> MAHHHHHHMSLAEFALIDRIRARTLERDDILLGIGDDAALLQPRANEQLVVTADTLNSGVHFPVETRAFDIGWKTLAVNLSDLAAMGARPAWCTLALSLPEASE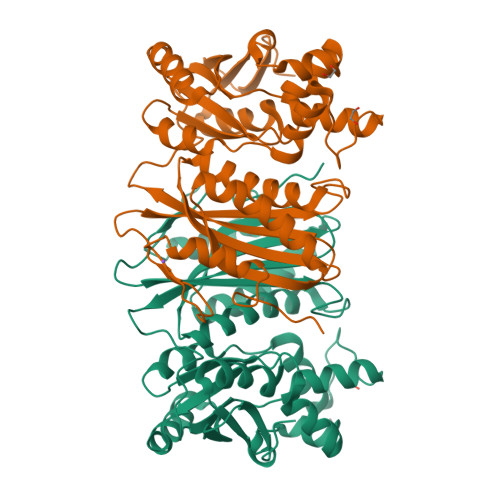DWIEAFGDGFFALADQHDIALIGGDTTRGPLSLSVTAMGQVGRGQALRRDRAQLGDDIWVSGTLGDAAGALRLWQQGALNLATATLLADYESLRLRLLRPTPRVTLGLRLRAFAHAAVDVSDGLLADLGHIAARSNVAAHVDADSLPISHALRELLGRDDARDCALRGGDDYELCFTAAADQRDALHYLAESLDLPLTRIGRIADGQGVHVDGEAADGGYQHFA>[2x]HMKADEMAHRRYCKRTI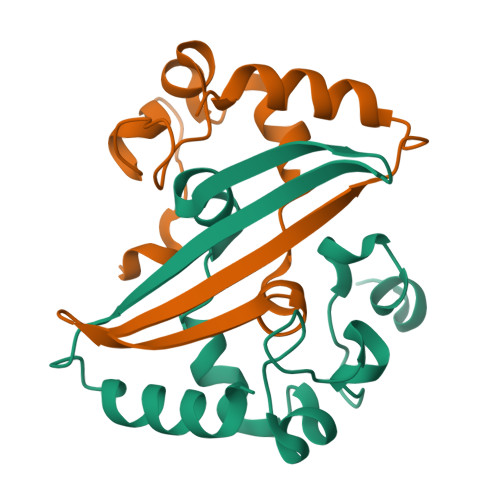PPNYRVDQVFGPRTKGKEGNFGDDKMNEEGIKDGRVTAMLNLVPSSHACLFGSRVTPKLQLDGLHLRFEFTTVVPCDDPQFDNYVKICDQCVDG>SGFSSEESSGRLTWRELLFGSGARKQSEAMKEEEIMMRLQEDSGAIFQRRSLTSKAALDPRLRCTEVDGNGNVIMVDGELKKSELIAKYGLLPRDLRKIDSSNLPHILVRPSAILINLLHLKVLIKHDRVLLFDVYGSTSSYPQSAFMYDLQGKLQQKQTGGANSLPYEFRALEAVLMSVTAELEADFEAVRDPVIRILSELEDDIDREKLRILLVLSKRVSTFEQKAKLVRDAIEELLEADDDLAAMYLTEKTHDLYRGEDDHTEVELLLESYHKLCDEVVQEASNLVSSIRNTEEIIRAILDANRNSLMLLDLKFSIGTLGLAMGTFLAGLYGMNLENFIEETNWGFGAITGLSTLLSLVVCWYGLAKLRKVQRVKMNGAGFTRHNHWFRDDSTDVLLDPSNRERLRKINMMKSHAKQKTAAAKKWPLNKL[5x]

The CorA/Mrs2 family of pentameric proteins are cardinal for the influx of Mg2+ across cellular membranes, importing the cation to mitochondria in eukaryotes. The mitochondrial inner membrane protein Mrs2 (mitochondrial RNA-splicing protein 2) is responsible for regulating the Mg2+ concentrations of mitochondria in eukaryotes, providing controlled uptake of the ion14–16. CorA/Mrs2 forms homopentamers with two transmembrane (TM) helices (TM1 and TM2) in each monomer, which are preceded by a soluble N-terminal domain (NTD) that regulates the Mg2+ passage. The protein family exposes only the loop between TM1 and TM2 to the surrounding environment but this stretch harbors a conserved selective filter GMN motif that is essential for permeation.

Consequently, to further illuminate the Mg2+ conductance mechanism, we prepared a new CtMrs2 sample using a mild isolation strategy with the inclusion of EDTA from cell lysis and until final usage. Two cryo-EM maps, with and without applied C5 symmetry, were determined at an overall resolution of 3.2 and 3.5 Å, respectively. The EDTA-induced structure preserves the homopentamer form. Indeed, the TM domain including the pore is well maintained overall and the intermembrane space remains negatively charged, presumably facilitating Mg2+ uptake. However, as partly achieved by rotation of these side chains away from the center (discussed below), the constriction rings of the pore marked by D420, M417–R413 and R406 in the closed structure display a striking enlargement of about 1, 5 and 13 Å. As a consequence, site S at the GMN motif is the narrowest point of the pore (4.0–4.7 Å in diameter) in the open structure. Thus, we conclude that this structure represents a conducting conformation, allowing the influx of partially hydrated Mg2+ to the matrix. Remarkably, among the most displaced structural features are the stalk and α5 helices of adjacent monomers, which are well separated in the open Mrs2 setting, thus eliminating the M1–M4 sites. However, while the conserved R314 has a peripheral orientation in the closed configuration, it serves as a wedge in between two adjacent stalk helices in the open conformation, through interaction with the invariant D410 and N414 of the neighboring monomer, thus directly influencing the matrix-facing end of the conducting pathway. Furthermore, toward the funnel tip, residues R200 and R203 of the conserved RDLR motif of the α1–α3 subdomain interact with E346, D348, E374 and E378 of the stalk helix of the adjacent monomer (side chain interactions except for E346), residues that assist in establishing the M1 and M2 sites in the closed structure. Interestingly, while we expected a Mg2+-depleted structure, we observed cryo-EM density at the S, P1 and P2 sites, which we tentatively assigned as Mg2+ despite the EDTA treatment of the sample (the P2 site is not as distinct as the other sites in the map calculated without imposed symmetry).> GGGHNVAWDYDNNVIRGVNLGGWFVLEPYMTPSLFEPFQNGNDQSGVPVDEYHWTQTLGKEAALRILQKHWSTWITEQDFKQISNLGLNFVRIPIGYWAFQLLDNDPYVQGQVQYLEKALGWARKNNIRVWIDLHGAPGSQNGFDNSGLRDSYNFQNGDNTQVTLNVLNTIFKKYGGNEYSDVVIGIELLNEPLGPVLNMDKLKQFFLDGYNSLRQTGSVTPVIIHDAFQVFGYWNNFLTVAEGQWNVVVDHHHYQVFSGGELSRNINDHISVACNWGWDAKKESHWNVAGEWSAAL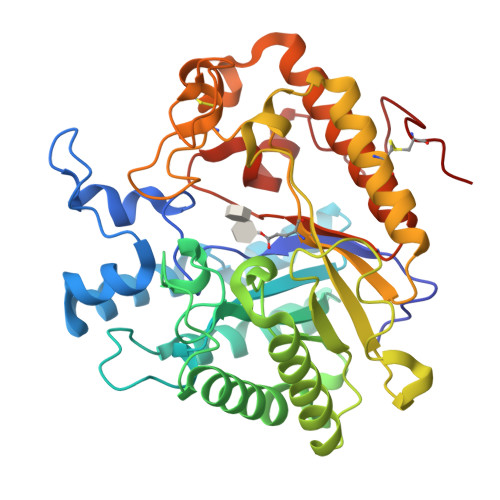TDCAKWLNGVNRGARYEGAYDNAPYIGSCQPLLDISQWSDEHKTDTRRYIEAQLDAFEYTGGWVFWSWKTENAPEWSFQTLTYNGLFPQPVTDRQFPNQCGFH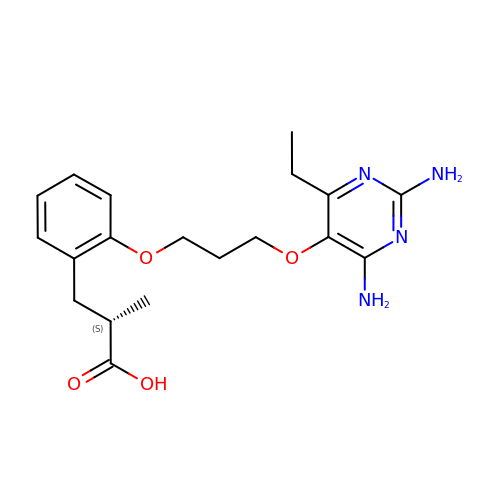(2S)-3-(2-{3-[(2,4-diamino-6-ethylpyrimidin-5-yl)oxy]propoxy}phenyl)-2-methylpropanoic acid | C19 H26 N4 O4 | ZLMWHEULHKTIRM-LBPRGKRZSA-N>MLLSNEEFLKKLTDLLQTHQSKGTGSVYLSQKCNPVDEGEGSSASVLIRAKSGAAEKISTVVELDYFTD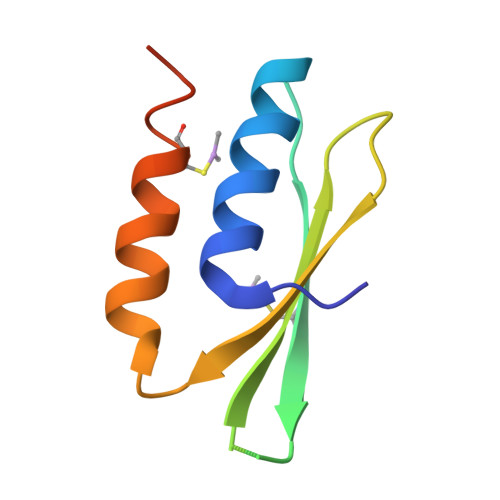FFQSYAEVCKGQIVGLKKRDRK[2x]>[4x]MSLFKIRMPETVAEGTRLALRAFSLVVAVDEHGGIGDGRSIPWNVPEDMKFFRDLTTKLRGKNVKPSPAKRNAVVMGRKTWDSIPPKFRPLPGRLNVVLSSTLTTQHLLDGLPDEEKRNLHADSIVAVNGGLEQALRLLASPNYTPSIETVYCIGGGSVYAEALRPPCVHLLQAIYRTTIRASESSCSVFFRVPESGTEAAAGIEWQRETISEELTSANGNETKYYFEKLIPRNREEEQYLSLVDRIIREGNVKHDRTGVGTLSIFGAQMRFSLRNNRLPLLTTKRVFWRGVCEELLWFLRGETYAKKLSDKGVHIWDDNGSRAFLDSRGLTEYEEMDLGPVYGFQWRHFGAAYTHHDANYDGQGVDQIKAIVETLKTNPDDRRMLFTAWNPSALPRMALPPCHLLAQFYVSNGELSCMLYQRSCDMGLGVPFNIASYALLTILIAKATGLRPGELVHTLGDAHVYSNHVEPCNEQLKRVPRAFPYLVFRREREFLEDYEEGDM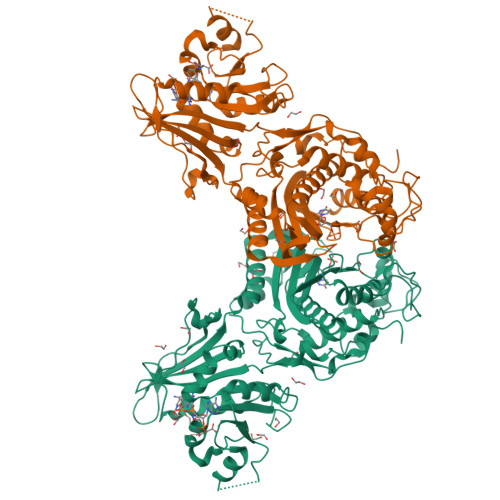EVIDYAPYPPISMKMAV> WSSTDKNFDNRPGVCFKVLTTKEPKANIKRCYNLPKTNNCLKCVLFVDA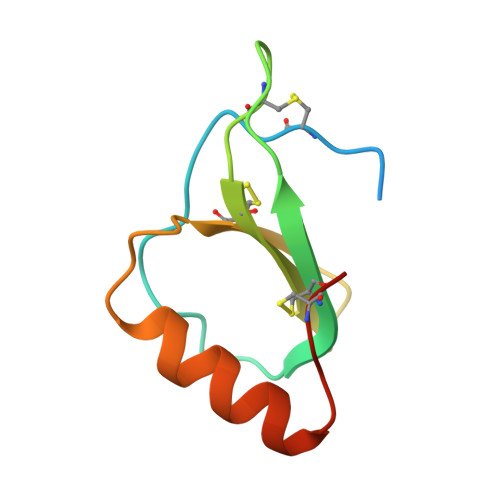SNRMKCIDPNASWLAERLYRLKEKGVTCRGEA>[4x]HHHHHHATLPAGASQVPTT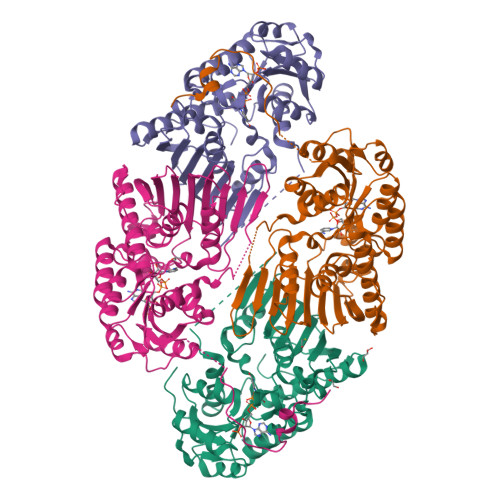PAGRPMPYAIRPMPEDRRFGYAIVGLGKYALNQILPGFAGCQHSRIEALVSGNAEKAKIVAAEYGVDPRKIYDYSNFDKIAKDPKIDAVYIILPNSLHAEFAIRAFKAGKHVMCEKPMATSVADCQRMIDAAKAANKKLMIGYRCHYDPMNRAAVKLIRENQLGKLGMVTTDNSDVMDQNDPAQQWRLRRELAGGGSLMDIGIYGLNGTRYLLGEEPIEVRAYTYSDPNDERFVEVEDRIIWQMRFRSGALSHGASSYSTTTTSRFSVQGDKAVLLMDPATGYYQNLISVQTPGHANQSMMPQFIMPANNQFSAQLDHLAEAVINNKPVRSPGEEGMQDVRLIQAIYEAARTGRPVNTDWGYVRQGGY> MRGSHHHHHHENLYFQGSLAVAEPVVNAADAKGTNVNDKVTASDFKLEKTAFDPNQSGNTFMAANFKVTGQVKSGDYFTAKLPDSVTGNGDVDYSNSNNTMPIADIKSTNGDVVAKATYDILT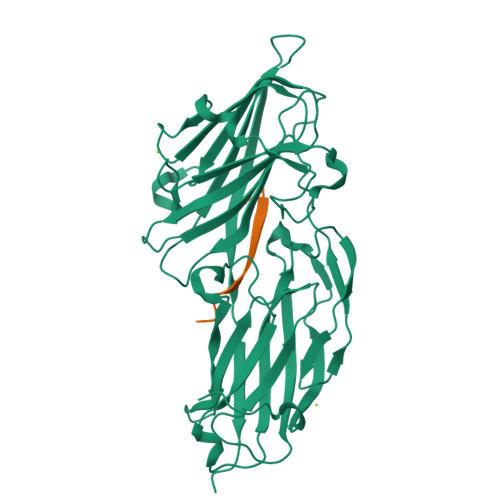KTYTFVFTDYVNDKENINGQFSLPLFTDRAKAPKSGTYDANINIADEMFDNKITYNYSSPIAGIDKPNGANISSQIIGVDTASGQNTYKQTVFVNPKQRVLGNTWVYIKGYQDKIEESSGKVSATDTKLRIFEVNDTSKLSDSYYADPNDSNLKEVTGEFKDKISYKYDNVASINFGDINKTYVVLVEGHYDNTGKNLKTQVIQENIDPATGKDYSIFGWNNENVVRYGGGSADGDSAVN;> GQSGSSGSGSNGD>[2x]HHHHHHSSGLVPRGSMPGRRKACFVTALTSRTELDIDPDKLRESVVELLERHPLVFEGTRQLALQHRPEA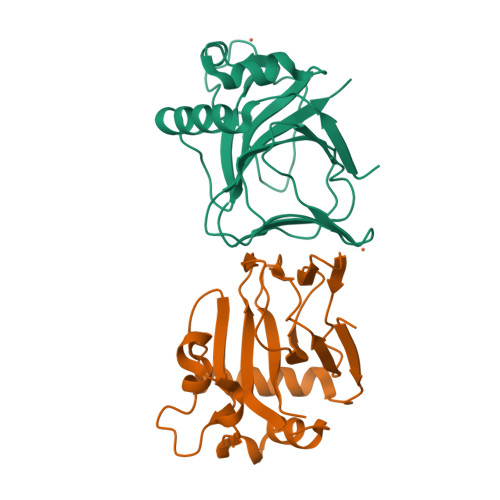TDPWYEGCQRQSLISSDSDFTEVHGELRDTYLGEVFDRLPFKPIRTRIMALDPKYCYSVHRALTPRYHLAVTTSEHARFVFIEHDKVLHIPADGDLYYVDTRQLHSAFNGGDDMRIHIVFGTDGESK> ALIICYYGKNGAVIGGDRRQIFFRGSEENRKILEEKLYSGEIKSEEELYKLAEKLNIKIIIEDDREKVRKISDSVVCGEVRSLGIDAKRRRVYATKGKCAIVDILNDTVTNQ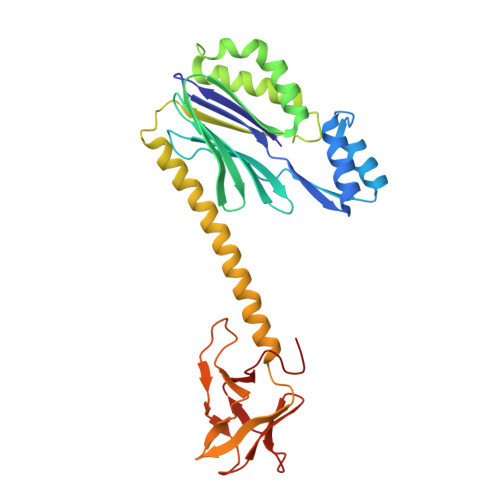TIKEGFGIVVLGNRFLKKKAEEELKRTAKLFPMMPIQQIEDAIKEIFEKLKWHPTVSKEYDIYSVNKYEKNFEEVIKKDIESLFKYREQLRKQLIDFGKVMSIVNKIVKNGEIGVIKDGKLHLYDDYIAIDKIDPNPKVFKVVDVEGNFKDGDIVVIENGDMKIKGTNEKVTTKYIIIHKGSHHHHHH> KDGDQCETSPCQNQGKCKDGLGEYTCTCLEGFEGKNCELFTRKLCSLD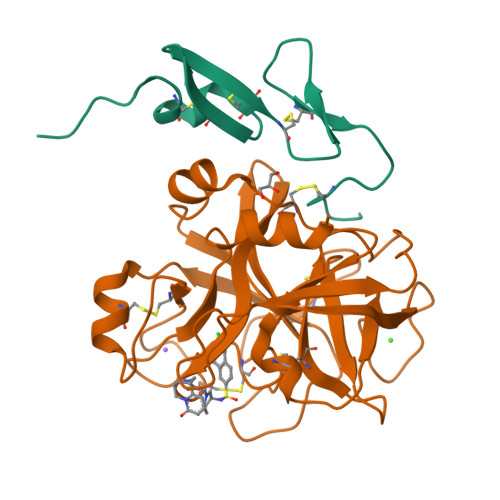NGDCDQFCHEEQNSVVCSCARGYTLADNGKACIPTGPYPCGKQTLE;> IVGGQECKDGECPWQALLINEENEGFCGGTILSEFYILTAAHCLYQAKRFKVRVGDRNTEQEEGGEAVHEVEVVIKHNRFTKETYDFDIAVLRLKTPITFRMNVAPACLPERDWAESTLMTQKTGIVSGFGRTHEKGRQSTRLKMLEVPYVDRNSCKLSSSFIITQNMFCAGYDTKQEDACQGDSGGPHVTRFKDTYFVTGIVSWGEGCARKGKYGIYTKVTAFLKWIDRSMKTRGLP>[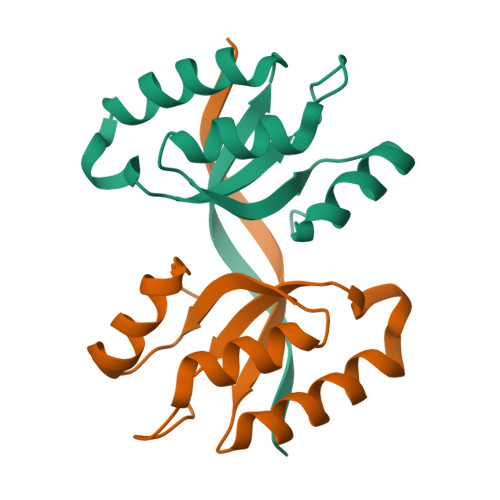2x]GAMGSTPIELKGSSFTLSVVHLHEAEPKVIHQALEDKIAQAPAFLKHAPVVLNVSALEDPVNWSAMHKAVSATGLRVIGVSGCKDAQLKAEIEKMGLPILTEG>QQDWLTFQKKHITNTRDVDCDNIMSTNLFHCKDKNTFIYSRPEPVKAICKGIIASKNVLTTSEFYLSDCNVTSRPCKYKLKKSTNKFCVTCENQAPVHFVGVGSC[2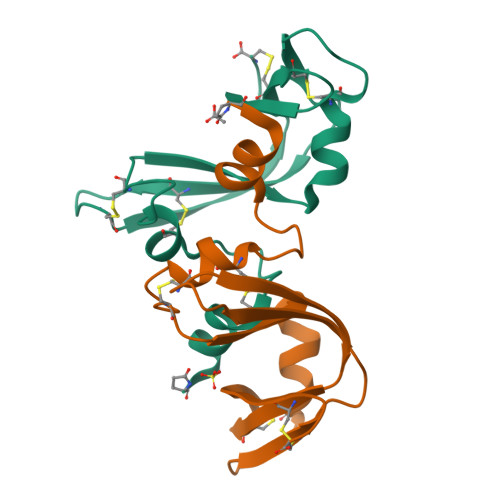x]Acanthamoeba sterol 14α-demethylase (CYP51) is an essential enzyme of the sterol biosynthetic pathway. Here, we report catalytic properties, inhibition, and structural characterization of CYP51 from Acanthamoeba castellanii. The enzyme displays a 100-fold substrate preference for obtusifoliol over lanosterol, supporting the plant-like cycloartenol-based pathway in the pathogen. Cys434 serves as the fifth (proximal) axial ligand to the heme iron.

VT1161 was selected for cocrystallization because, in this work, it was found to be the most potent inhibitor of Acanthamoeba sp. Additionally, it has been previously shown that VT1161 does not bind to human CYP51,59 indicating the desired selectivity. The asymmetric unit consisted of six very similar protein molecules, with the average RMSD between their Cα atoms being 0.22 Å. Each protein molecule contained one molecule of the inhibitor bound in essentially the same conformation, except for some rotations of the very distal portion of its long arm (trifluoroethoxy group). Within the active site, the N4 nitrogen of the VT1161 tetrazole ring forms a 2.2 Å-long coordination bond with the heme iron. Due to the lack of helices A and A′ in the structure, the trifluoroethoxy group of VT1161 is partially exposed to the solvent and has a higher B-factor (up to 90 A2 vs 8–10 A2 for the tetrazole and β-phenyl rings inside the active site). At van der Waals distances (<4.6 Å), the inhibitor is contacted by 16 mainly hydrophobic amino acid residues. The positions of most of these residues are similar to those in the structure without a bound inhibitor, except for Phe293 and Met471, which adopt different conformations, and Tyr114, whose side chain ring rotates ∼ 90° yet does not lose its H-bond with the heme. Overall, the binding of VT1161 did not cause any substantial rearrangements in the protein backbone. Thus, the strong inhibitory effect of VT1161 on the activity of A. castellanii CYP51 does not appear to be a result of some inhibitor-induced large-scale conformational change in the enzyme. We surmise that, instead, multiple interactions between VT1161 and the protein moiety impede the conformational rearrangements that are required for catalysis (e.g., acquiring the substrate, redox partner recognition).

>[6x]MAKKTSSKGKLPPVVSSLIPFVGSGLSFAGGPLQYTTDAYKKYGDIFTMKVFGQRLTFLVGPDAHVPFFSQGDAELSQDEPYQFSVPIFGPNVVYGADLAHRNQQLKFIAASLSTKALQSYVPLIVKEAEDFFAKWDKSGTVDIRDALAELIILTASRCLMGKEIRENLFTEVAKLYQTLDEGLLPISVFFPYLPIPAHKRRDEARLAMVRMFKKIIDERRANPEVKHNDCLQVFMDARYRGEEQALNDEEITGLMIALLFAGQHTSSVTGSWTGLLLFEANNKKKFLPGVLEEQEEIRKEFGDELTMEALNKMDKLHRCVKEALRMYPPLLFVMRKVIKPFSYKDYYVPEGDTVFVSPALSMRVEEVFPNADQYNPERFVEEDKQAQKYRFVGFGAGRHGCMGENFAYLQIKTIWSVLLRNFDIELVGELPKPDYTAMVVGPAHPCLLRYTRKHHHHHH>MGSSHHHHHHSSGPQQGLRQHNNPFGNALIPDMIADASIQEINGVFYCYATTDGYGQGLKTSGPPVVWKSKDFVHWSFDGTYFPSAAKEKYWAPSKAIFANGKYYIYPTINGYMYPAVADKPEGPFKLARGKDEFYKPFTPSTLLQSKNPGGIDAEIFVDDDGQAYVFWGRRHVAKLNEDMITVDSVVQVISTPRKEYSEGPIFFKRKGIYYYLYTIGGDEKYQYAYVMSRVSPMGPFEAPEQDIISTTNYERGIFGPGHGCVFHPEGTDNYYFAYLEFGRRSTNRQTYVNQLKFNEDGTIRPVELTMDGVGALKKVKSDKKMKIDTVYASSIEVPLKIEPMKDPTCLRTEYFVPSFAVDGANGSRWMAAAEDSINPWIVADLGTVKKVRRSEIYFV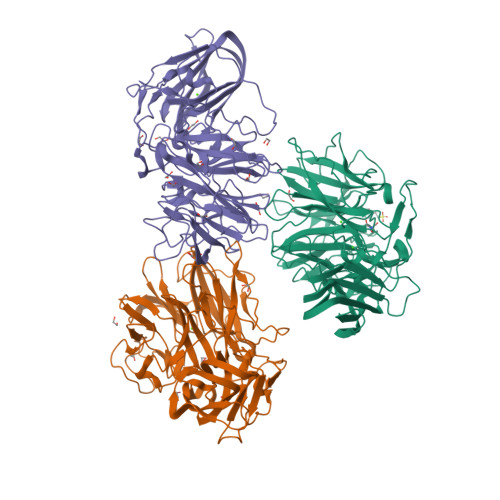RPTAGHAYVIEASMDGKVWQEFAVHQDRKMCSPHTDVLNKRFRYLRIKILKGVPGIWEWNIY[3x]> YEHTAVMPNKVGIPYKALVERPGYAPVHLQIQLVNTRIIPSTNLEYITCKYKTKVPSPVVKCCGATQCTSKPHPDYQCQVFTGVYPFMWGGAYCFCDTENTQMSEAYVERSEECSIDHAKAYKVHTGTVQAMVNITYGSVSWRSADVYVNGETPAKIGDAKLIIGPLSSAWSPFDNKVVVYGHEVYNYDFPEYGTGKAGSFGDLQSRTSTSNDLYANTNLKLQRPQAGI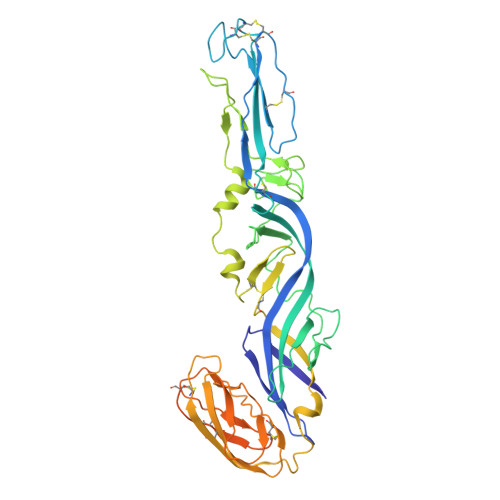VHTPFTQAPSGFERWKRDKGAPLNDVAPFGCSIALEPLRAENCAVGSIPISIDIPDAAFTRISETPTVSDLECKITECTYASDFGGIATVAYKSSKAGNCPIHSPSGVAVIKENDVTLAESGSFTFHFSTANIHPAFKLQVCTSAVTCKGDCKPPKDHIVDYPAQHTESFTSAISATAWSWLKVLVGGTSAFIVLGLIATAVVALVLFFHRH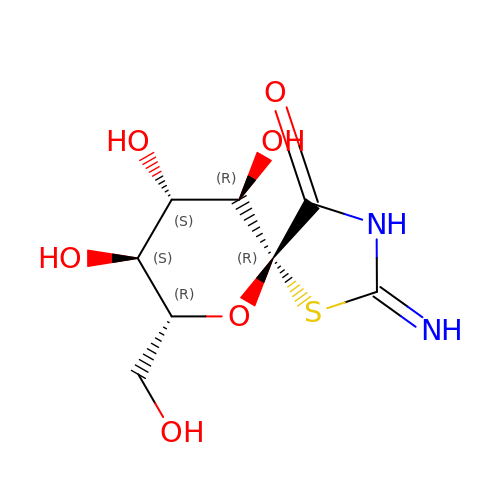(5R,7R,8S,9S,10R)-8,9,10-trihydroxy-7-(hydroxymethyl)-2-imino-6-oxa-1-thia-3-azaspiro[4.5]decan-4-one | C8 H12 N2 O6 S | UADFNVXVJZELQM-UXDJRKLDSA-N Acylpeptide hydrolase (APEH) or acylaminoacyl‐peptidase (AAP) is a serine hydrolase that regulates protein metabolism. It can also bind to and process unusual substrates, acting as a detoxifier. The most prominent physiological function of APEH is the removal of N‐acetylated amino acids from the N‐terminus of oligopeptides and proteins (Perrier et al., 2005) thereby exerting crucial control over the proteasomal degradation of damaged and misfolded proteins (Adibekian et al., 2011; Hoernstein et al., 2023; Hwang et al., 2010; Palmieri et al., 2011; Sandomenico et al., 2021; Shimizu et al., 2003; Shimizu et al., 2004; Tangri et al., 2021). The S9 serine protease subfamily, the so‐called oligopeptidases, employs a further, size‐based selection process (Kobayashi & Smith, 1987). Their active site is sequestered in an inner pocket that is formed between the catalytic hydrolase domain and a propeller domain that caps it.

Here we determined the tetrameric structure of pAPEH in complex with acetyl‐alanyl‐chloromethyl ketone (AcACMK), a covalent inhibitor using cryo‐EM with a maximum resolution of 3.19 Å. The AcACMK inhibitor hydrolyzed into acetyl‐alanyl‐methyl‐hemiketal (AcAMHK) and bound covalently to the active Ser587 and His707 of each monomer of the tetrameric pAPEH structure. The oxygen of the tetrahedral center (most likely an OH group in the stable form of the complex) is oriented by the oxyanion site—the backbone amides of Gly509 and His588—similarly to what is expected during catalysis, however, neither distance (3.9 and 3.6 Å, respectively) is close enough for the formation of a proper H‐bond. The amide NH moiety of AcAMHK points toward carbonyl oxygen of Gly509, which is—again—similar to those seen in substrate complexes of serine protease enzymes, but here it not quite close enough (3.8 Å) for a strong interaction. The acetyl group of AcAMHK is coordinated by the Nε‐atom of Arg677, which flips to fulfill this interaction (as compared to its position in the ligand‐free form of the enzyme). The small Ala sidechain of the inhibitor sits in the shallow, rather hydrophobic S1 binding pocket. Furthermore, the loop holding the catalytic His707 also shifts closer to the inhibitor by 0.5 Å, as measured at His707(Cα). Since in this case a covalent bond is established both toward the catalytic Ser and the catalytic His, both the His‐loop and the oxyanion‐loop move closer to the inhibitor (and each other), tightening all three dimensions of the active site. It seems as if the too spacious active site of the ligand‐free form would attempt to move closer to activate the enzyme sufficiently for binding the inhibitor, but the resultant active site pocket still seems quite a bit looser than in the case of the canonical binding mode.

>MERQVLLSEPEEAAALYRGLSRQPALSAACLGPEVTTQYGGRYRTVHTEWTQRDLERMENIRFCRQYLVFHDGDSVVFAGPAGNSVETRGELLSRESPSGTMKAVLRKAGGTGTAEEKQFLEVWEKNRKLKSFNLSALEKHGPVYEDDCFGCLSWSHSETHLLYVADKKRPKAESFFQTKALDVTGSDDEMARTKKPDQAIKGDQFLFYEDWGENMVSKSTPVLCVLDIESGNISVLEGVPESVSPGQAFWAPGDTGVVFVGWWHEPFRLGIRFCTNRRSALYYVDLTGGKCELLSDESVAVTSPRLSPDQCRIVYLRFPSLVPHQQCGQLCLYDWYTRVTSVVVDIVPRQLGEDFSGIYCSLLPLGCWSADSQRVVFDSPQRSRQDLFAVDTQMGSVTSLTAGGSGGSWKLLTIDRDLMVVQFSTPSVPPSLKVGFLPPAGKEQAVSWVSLEEAEPFPDISWSIRVLQPPPQQEHVQYAGLDFEAILLQPSNSPEKTQVPMVVMPHGGPHSSFVTAWMLFPAMLCKMGFAVLLVNYRGSTGFGQDSILSLPGNVGHQDVKDVQFAVEQVLQEEHFDAGRVALMGGSHGGFLSCHLIGQYPETYSACVVRNPVINIASMMGSTDIPDWCMVEAGFSYSSDCLPDLSVWAAMLDKSPIKYAPQVKTPLLLMLGQEDRRVPFKQGMEYYRVLKARNVPVRLLLYPKSTHALSEVEVESDSFMNAVLWLCTHLGS[4x]> MAKLNLAVLNNVFSELLTQEINRSATFLGLLSKYPERKSNIQWGVGMGGTTATGVAITGSAPAASMDATLPAQLPISAASVQSTFTLNLKEIEESKEQVTNEELRNLLEAQMRNAVEEIATTLNKKLYDGSGAIADGGLIGLSIAASGQDYAGISSATYPLWNVSEVDAWDANATGTDKRQAL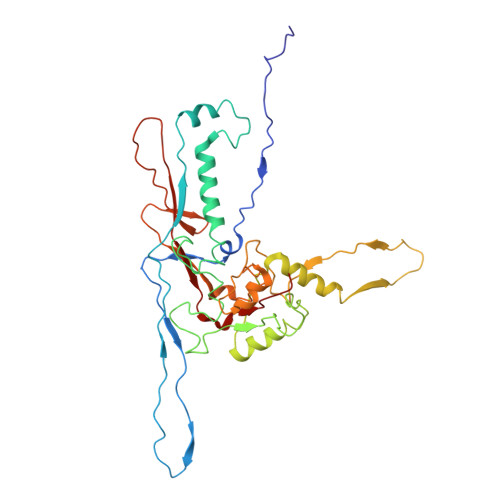KTDFMLELDRKIRYRPGAYDLILTTPKVVEQYKKVFEANRSYQIMTFDGQRVPLIDLGFNVAGYMGRPIIDDVFCSRTRTAAESAITTALGTAVDEGVMYFLKKDDLRFYSTPVVGAFSANGVYTLMRQLAQTSLYVDNFVVGCIPQLQLTTRKNVGVIKNIKVG> MALSE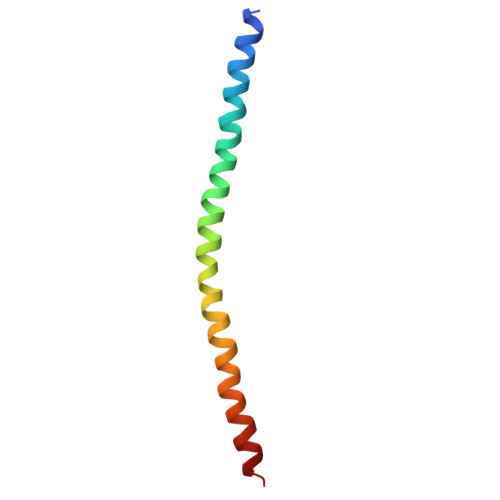IETRHSEIIKLENSIRELHDMFMDMAMLVESQGEMIDRIEYNVEHAVDYVERAVSDTKKAVK>ASMGKSAVIFVERATPATLTELKDALSNSILSVRDPWSIDFRTYRCSIKNLPADVSKLMYSITFHHHGRQTVLIKDNSAMVTTAAAADIPPALVFNGSSTGVPESIDTILSSKLSNIWMQRQLIKGDAGETLILDGLTVRLVNLFSSTGFKGLLIELQADEAGEFETKIAGIEGHLAEIRAKEYKTSSDSLGPDTSNEICDLAYQYVRALEL[4x];>[4x]VQQLSLFGSIGDDGYDLLISTLTTISGNPPLLYNSLCTVWKP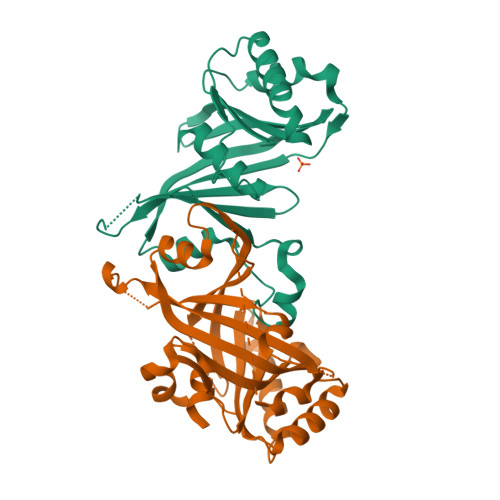NPSYDVENVNSRNQLVEPNRIKLSKEVPFSYLIDETMMDKPLNFRILKSFTNDKIPLNYAMTRNILHNTVPQVTNFNSTNEDQNNSKHTEDTVNESRNSDDIIDVDMDASPAPSNESCSPWSLQISDIPAAGNNRSVSMQTIAETIILSSAGKNSSVSSLMNGLGYVFEFQYLTIGVKFFMKHGLILELQKIWQIEEAGNSQITSGGFLLKAYINVSRGTDIDRINYTETVLMNLKKELQGYIELSVPDRQSMDSRVAHGNILIAAALEHHHHHH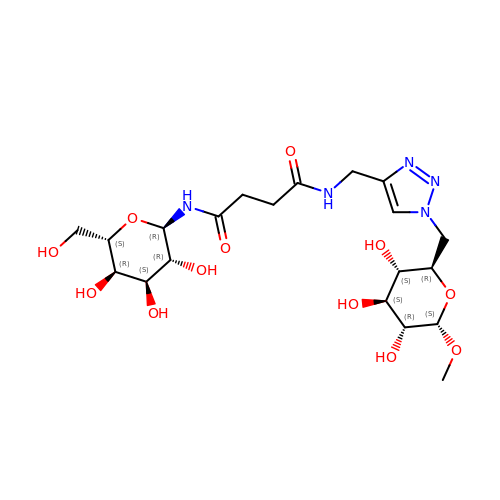N-[(2R,3R,4S,5R,6S)-3,4,5-trihydroxy-6-(hydroxymethyl)tetrahydro-2H-pyran-2-yl]-N'-[(1-{[(2R,3S,4S,5R,6S)-3,4,5-trihydroxy-6-methoxytetrahydro-2H-pyran-2-yl]methyl}-1H-1,2,3-triazol-4-yl)methyl]butanediamide | C20 H33 N5 O12 | ZVODTTTYSJJUKY-SRYZRXLVSA-N> GAMAVALLGSLAACGGSKEPTTTADGKPIVSVLVVKRPATDKIANMQWAKDLEADCDCKIEWQEVSEDAWAQQKNATLAAGKIADVSLHAFFPANAAQFPGLFEDLSKDLDKMPNVKQFFKEKPDAQKLTTDPEGHMYALPSSRGKSYSGTGQHMFINKTWLDKLGLQVPTTWDELENVLKAFKTEDPNGNGQADEIPMNIRKLDSYFTYYSPMLLLNSTGIVTGFNKGASPTGFYAKNGVVKSFLTSDEYKQVIKYYHKLISEGLIPADWATKTFDACDTDQLSDGKTAKTGVSFGWSQDA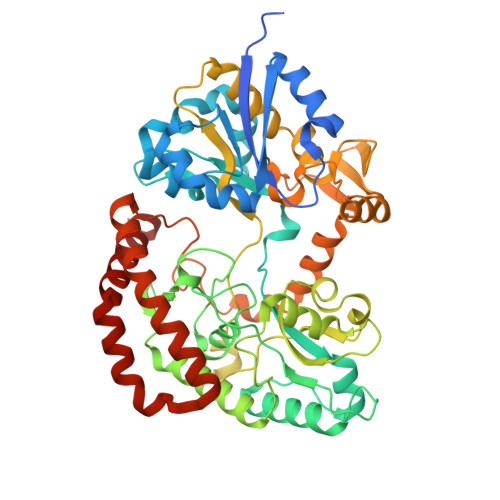SFGTLKDQYIPIPVPSAPGVSPDKTVWDGSSAEFEADRFSLSSHAANKDAALKLANLLYSEKYSVQQFLGSFGNLVTDDGNRHYTVDEDKYTKAMGDNLFPGLADRFSGWIPDGVTIKGDVDGDNLLEANKPYEEQRSHFDPVKDYIPDYVNPDPTDSNTLTNNNAQISNVVMQKTATWMSKGGIDEEWDAYCKQLDSLGLQENVKIWQKWYDIYTKK>GMSKVEQNAQHNIQQTSPNAAVQSGLQEWHRIIAEADWERLPDLLAEDVVFSNPSTFDPYHGKGPLMVILPAVFSVLENFQYARHFSSKSGYVLEFNANMGDELLTGVDLIEFNDAGKITDLVVMMRPASVVIDLSV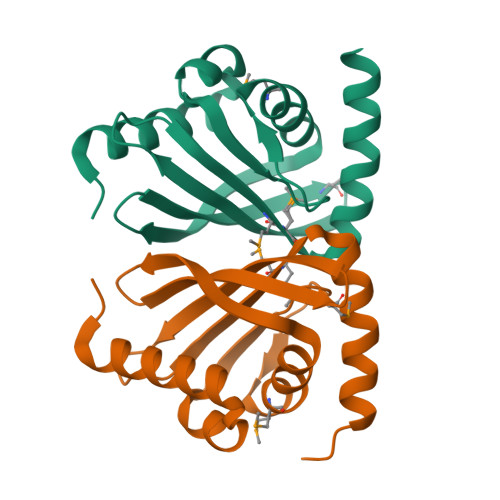EVGKRIAAAQS[4x]>MAKDIGINSDPNSSSVDKLMKSSGVSNPTYTLVWKVWILAVTLYYAIRIPLTLVFPSLFSPLLPLDILASLALIADIPLDLAFESRRTSGRKPTLLAPSRLPDLLAALPLDLLVFALHLPSPLSLLSLVRLLKLISVQRSATRILSYRINPALLRLLSLVGFILLAAHGIACGWMSLQPPSENPAGTRYLSAFYWTITTLTTIGYGDITPSTPTQTVYTIVIELLGAAMYGLVIGNIASLVSKLDAAKLLHRERVERVTAFL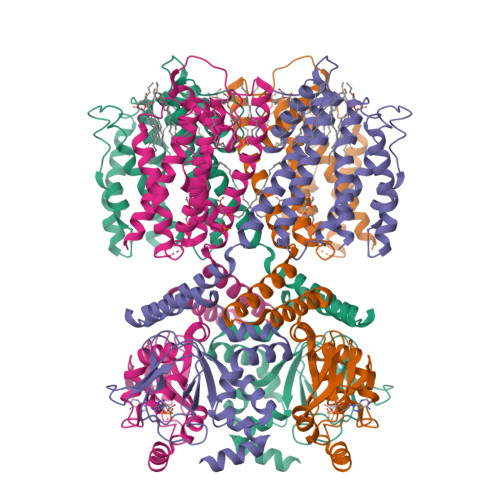SYKRISPELQRRIIEYFDYLWETRRGYEEREVLKELPHPLRLAVAMEIHGDVIEKVPLFKGAGEEFIRDIILHLEPVIYGPGEYIIRAGEMGSDVYFINRGSVEVLSADEKTRYAILSEGQFFGEMALILRAPRTATVRARAFCDLYRLDKETFDRILSRYPEIAAQIQELAVRRKELESSGLVPRGSVKHHHH[4x]>MQSVDVAIVGGGMVGLAVACGLQGSGLRVAV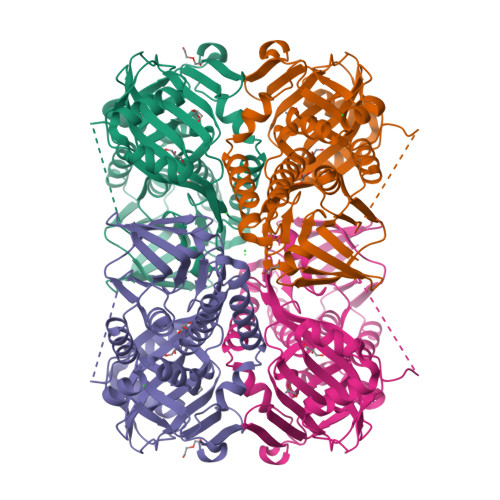LEQRVQEPLAANAPPQLRVSAINAASEKLLTRLGVWQDILSRRASCYHGMEVWDKDSFGHISFDDQSMGYSHLGHIVENSVIHYALWNKAHQSSDITLLAPAELQQVAWGENETFLTLKDGSMLTARLVIGADGANSWLRNKADIPLTFWDYQHHALVATIRTEEPHDAVARQVFHGEGILAFLPLSDPHLCSIVWSLSPEEAQRMQQASEDEFNRALNIAFDNRLGLCKVESARQVFPLTGRYARQFASHRLALVGDAAHTIHPLAGQGVNLGFMDAAELIAELKRLHRQGKDIGQYIYLRRYERSRKHSAALMLAGMQGFRDLFSGTNPAKK[2x]> PKYTIVDKETCIACGACGAAAPD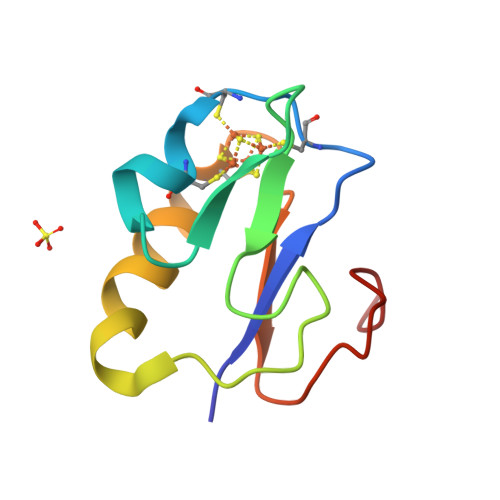IYDYDEDGIAYVTLDDNQGIVEVPDILIDDMMDAFEGCPTDSIKVADEPFDGDPNKFE> MRVLVVEDNALLRHHLKVQIQDAGHQVDDAEDAKEADYYLNEHIPDIAIVDLGLPDEDGLSLIRRWRSNDVSLPILVLTARESWQDKVEVLSAGADDYVTKPFHIEEVMARMQALMRRN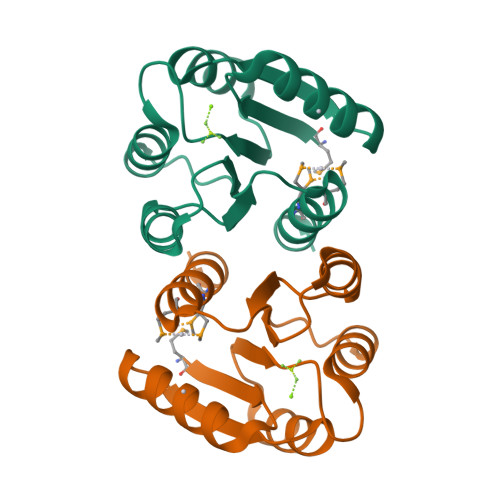SQ(2~{S})-2-[[(2~{S})-4-methyl-1-oxidanyl-1-oxidanylidene-pentan-2-yl]carbamoyloxy]pentanedioic acid | C12 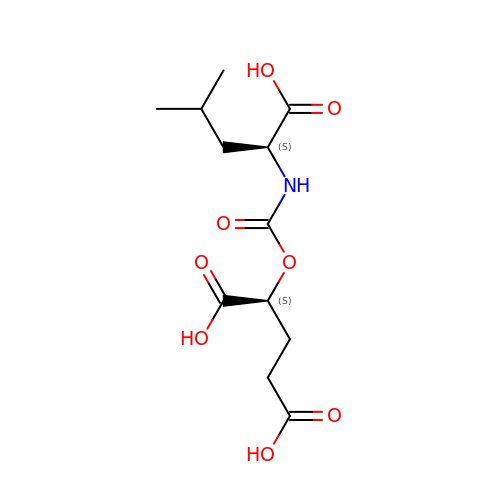H19 N O8 | WQDZXAWSGIQGKR-YUMQZZPRSA-N> LLKSFKTEINPSEEQKVKIHKTIGTCRFIYNFYLAHNKELYDKGEKFMSGKSFSVWLNNEYLPQNPDKLWIKEVSSKSVKHSIENGCIAFTRFFKHQSAFPNLKKKGKSDVKMYFVKNNPKDCRCERHRINIPSLGWVRIKEKGYIPTTKDGYVIKSGTVSMKADRYYVSVLVEISNNKIANNSNAGIGIDLGLKDFAIVSNGKTYKNINKSARLKKHEKQLIREQRSLSRKYENLKKGESTQKANIQKQRLKVQKLHHRMDNIRTDYINKTIAEIVKTKPSYITIEDLNVKGMMKNRHLSKAVASQKFYEFRTKLQAKCNENGIELRVVDRWYPSSKTCHCCGAVKKDLKLSDRIFKCSCGYVEDRAFNAALNLRDAITYEVA

TnpB is a RuvC domain-containing protein and predicted to be an ancestor of the Cas12 nucleases of CRISPR-Cas systems. Our biochemical data demonstrate that RAGATH-18-derived RNA (reRNA) interact with IS607 TnpB to form a novel programmable reRNA-guided DNase system. To the best of our knowledge, these IS607 TnpBs with an average size of 390 aa (330–433 aa) represent the smallest programmable endonucleases with activity in human cells identified thus far.

We determined the structure of a ternary complex comprising ISFba1 TnpB (D371A catalytic mutant), a 207-nt reRNA containing a 20-nt guide segment, a 36-nt target DNA strand and a 20-nt non-target DNA strand with a 5’-AGGAG TAM using cryo-EM at resolution of 3.0 Å. The structure revealed that ISFba1 TnpB and reRNA form a complex with 1:1 stoichiometry. ISFba1 TnpB consists of an amino-terminal TAM-interacting domain (TID) and a non-target-strand recognition (REC1) domain, a target-strand recognition (REC2) domain, a reRNA-binding domain (RBD), and a RuvC domain at its carboxy-terminus. The guide RNA–target DNA heteroduplex binds to the central channel formed by TID and REC1 from one side, and the REC2 and RuvC domains from the other side. In ISFba1 TnpB system, the reRNA plays a scaffolding role in organizing the complex via stabilizing the conformation of the ISFba1 TnpB effector protein for targeting the dsDNA substrate. The REC2 (residues R227, R230, R234, N238 and N249), RuvC (residues K299, N300 and R301) and RBD (residues K341 and K354) domains pack against the sugar-phosphate backbone of the reRNA at one side, whereas TID is anchored on SL3 of the 3’ flanking and 5’ flanking motifs of the reRNA through polar interactions via R130, R132 and R142. The 5’-AGGAG TAM-containing duplex is specifically recognized by REC1 and TID. The nucleobases of dG(–1*), dG(–4*) and dA(–5*) of TAM form hydrogen-bonding interactions with K83, N121 and N122 of TID, respectively. The TAM-proximal end (base pairs 1–7) of the heteroduplex is recognized by the REC1 and RuvC domains, whereas the middle portion (base pairs 8–14) of the heteroduplex is bound by the REC2 domain. In this regard, our structural observation revealed that, as compared with Cas9, the reduced contacts between RNA–DNA heteroduplex and the REC domain of ISFba1 TnpB support that ISFba1 TnpB may target a dsDNA substrate stringently despite its miniature size.> MRETHLRSILHTIPDAMIVIDGHGIIQLFSTAAERLFGWSELEAIGQNVNILMPEPDRSRHDSYISRYRTTSDPHIIG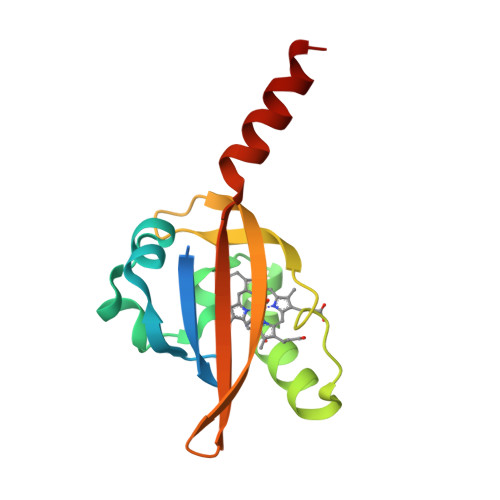IGRIVTGKRRDGTTFPMHLSIGEMQSGGEPYFTGFVRDLTEHQQTQARLQELQ> MSNTEELIQNSIGFLQKTFKALPVSFDSIRHEPLPSSMLHASVLNFEWEPLEKNISAIHDRDSLIDIILKRFIIDSMTNAIEDEEENNLEKGLLNSCIGLDFVYNSRFNRSNPASWGNTFFELFSTIIDLLNSPSTFLKFWPYAESRIEWFKMNTSVEPVSLGESNLISYKQPLYEKLRHWNDILAKLENNDILNTVKHYNMKYKLENFLSELLPINEESNFNRSASISALQESDNEWNRSARERESNRSSDVIFAADYNFVFYHLIICPIEFAFSDLEYKNDVDRSLSPLLDAILEIEENFYSKIKMNNRTRYSLEEALNTEYYANYDVMTPKLPVYMKHSNAMKMDRNEFWANLQNIKESDDYTLRPTIMDISLSNTTCLYKQLTQEDDDYYRKQFILQLCFTTNLIRNLISSDETRNFYKSCYLRENPLSDIDFENLDEVNKKRGLNLCSYICDNRVLKFYKIKDPDFYRVIRKLMSSDEKFTTAKIDGFKEFQNFRISKEKIPPPAFDETFKKFTFIKMGNKLINNVWKIPTGLDKIEQEVKKPEGVYEAAQAKWESKISSETSGGEAKDEIIRQWQTLRFLRSRYLFDFDKVNEKTGVDGLFEEPRKVEALDDSFKEKLLYKINQEHRKKLQDAREYKIGKERKKRALEEEASFPEREQKIKSQRINSASQTEGDELKSEQTQPKGEISEENTKIKSSEVSSQDPDSGVAGEFAPQNTTAQLENPKTEDNNAATSNISNGSSTQDMK;> MAEQTLLSKLNALSQKVIPPASPSQASILTEEVIRNWPERSKTLCSDFTALESNDEKEDWLRTLFIELFDFINKNDENSPLKLSDVASFTNELVNHERQVSQASIVGKMFIAVSSTVPNINDLTTISLCKLIPSLHEELFKFSWISSKLLNKEQTTLLRHLLKKSKYELKKYNLLVENSVGYGQLVALLILAYYDPDNFSKVSAYLKEIYHIMGKYSLDSIRTLDVILNVSSQFITEGYKFFIALLRKSDSWPSSHVANNSNYSSLNEGGNMIAANIISFNLSQYNEEVDKENYERYMDMCCILLKNGFVNFYSIWDNVKPEMEFLQEYIQNLETELEEESTKGVENPLAMAAALSTENETDEDNALVVNDDVNMKDKISEETNADIESKGKQKTQQDILLFGKIKLLERLLIHGCVIPVIHVLKQYPKVLYVSESLSRYLGRVFEYLLNPLYTSMTSSGESKDMATALMITRIDNGILAHKPRLIHKYKTHEPFESLELNSSYVFYYSEWNSNLTPFASVNDLFENSHIYLSIIGPYLGRIPTLLSKISRIGVADIQKNHGSESLHVTIDKWIDYVRKFIFPATSLLQNNPIATSEVYELMKFFPFEKRYFIYNEMMTKLSQDILPLKVSFNKAEREAKSILKALSIDTIAKESRRFAKLISTNPLASLVPAVKQIENYDKVSELVVYTTKYFNDFAYDVLQFVLLLRLTYNRPAVQFDGVNQAMWVQRLSIFIAGLAKNCPNMDISNIITYILKTLHNGNIIAVSILKELIITVGGIRDLNEVNMKQLLMLNSGSPLKQYARHLIYDFRDDNSVISSRLTSFFTDQSAISEIILLLYTLNLKANTQNSHYKILSTRCDEMNTLLWSFIELIKHCLKGKAFEENVLPFVELNNRFHLSTPWTFHIWRDYLDNQLNSNENFSIDELIEGAEFSDVDLTKISKDLFTTFWRLSLYDIHFDKSLYDERKNALSGENTGHMSNRKKHLIQNQIKDILVTGISHQRAFKKTSEFISEKSNVWNKDCGEDQIKIFLQNCVVPRVLFSPSDALFSSFFIFMAFRTENLMSILNTCITSNILKTLLFCCTSSEAGNLGLFFTDVLKKLEKMRLNGDFNDQASRKLYEWHSVITEQVIDLLSEKNYMSIRNGIEFMKHVTSVFPVVKAHIQLVYTTLEENLINEEREDIKLPSSALIGHLKARLKDALELDEFCTLTEEEAEQKRIREMELEEIKNYETACQNEQKQVALRKQLELNKSQRLQNDPPKSVASGSAGLNSKDRYTYSRNEPVIPTKPSSSQWSYSKVTRHVDDINHYLATNHLQKAISLVENDDETRNLRKLSKQNMPIFDFRNSTLEIFERYFRTLIQNPQNPDFAEKIDSLKRYIKNISREPYPDTTSSYSEAAAPEYTKRSSRYSGNAGGKDGYGSSNYRGPSNDRSAPKNIKPISSYAHKRSELPTRPSKSKTYNDRSRALRPTGPDRGDGFDQRDNRLREEYKKNSSQRSQLRFPEKPFQEGKDSSKANPYQASSYKRDSPSENEEKPNKRFKKDETIRNKFQTQDYRNTRDSGAAHRANENQRYNGNRKSNTQALPQGPKGGNYVSRYQR;> MSTIGAVDILNQKTITSEVAASVTSKYLQSTFSKGNTSHIEDKRFIHVSSRSHSRFTSTPITPNEILSLKFHVSGSSMAYSRMDGSLTVWFIKDASFDKSVEVYIPDCCGSDKLATDLSWNPTSLNQIAVVSNSSEISLLLINEKSLTASKLRTLSLGSKTKVNTCLYDPLGNWLLAATKSEKIYLFDVKKDHSSVCSLNISDISQEDNDVVYSLAWSNGGSHIFIGFKSGYLAILKAKHGILEVCTKIKAHTGPITEIKMDPWGRNFITGSIDGNCYVWNMKSLCCELIINDLNS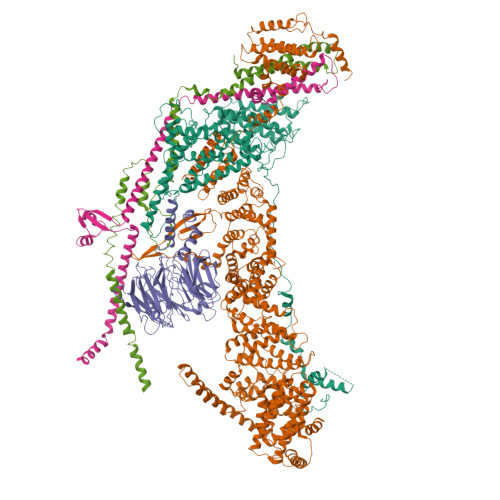AVTTLDVCHLGKILGICTEDEMVYFYDLNSGNLLHSKSLANYKTDPVLKFYPDKSWYIMSGKNDTLSNHFVKNEKNLITYWKDMFDNTMIEKRRKNNGGGNNHNKRTSKNTDRIGKDRPSRFNSKK;> MPLSQKQIDQVRTKVHYSEVDTPFNKYLDILGKVTKLTGSIINGTLSNDDSKIEKLTEQNISQLKESAHLRFLDLQSSIDTKKVADENWETCQQETLAKLENLKDKLPDIKSIHSKLLLRIGKLQGLYDSVQVINREVEGLSEGRTSLVVTRAEWEKELGTDLVKFLIEKNYLKLVDPGLKKDSSEERYRIYDDFSKGPKELESINASMKSDIENVRQEVSSYKEKWLRDAEIFGKITSIFKEELLKRDGLLNEAEGDNIDEDYESDEDEERKERFKRQRSMVEVNTIENVDEKEESDHEYDDQEDEENEEEDDMEVDVEDIKEDNEVDGESSQQEDNSRQGNNEETDKETGVIEEPDAVNDAEEADSDHSSRKLGGTTSDFSASSSVEEVK;> MTKEEGRTYFESLCEEEQSLQESQTHLLNILDILSVLADPRSSDDLLTESLKKLPDLHRELINSSIRLRYDKYQTREAQLLEDTKTGRDVAAGVQNPKSISEYYSTFEHLNRDTLRYINLLKRLSVDLAKQVEVSDPSVTVYEMDKWVPSEKLQGILEQYCAPDTDIRGVDAQIKNYLDQIKMARAKFGLENKYSLKERLSTLTKELNHWRKEWDDIEMLMFGDDAHSMKKMIQKIDSLKSEINAPSESYPVDKEGDIVLE> GSHMASHKKKGCVVIVGRINLSGDTAYAQQTRGEEGTQETSQTGRDKNVVTGEVQVLSTA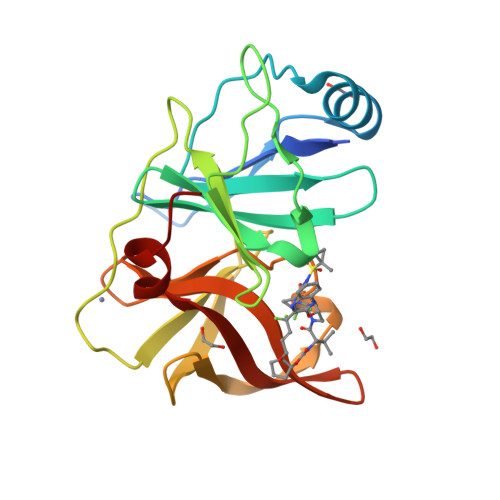TQTFLGTTVGGVIWTVYHGAGSRTLAGAKHPALQMYTNVDQDLVGWPAPPGAKSLEPCACGSSDLYLVTRDADVIPARRRGDSTASLLSPRPLAYLKGSSGGPVMCPSGHVAGIFRAAVSTRGVAKSLQFIPVETLSTQARSP>[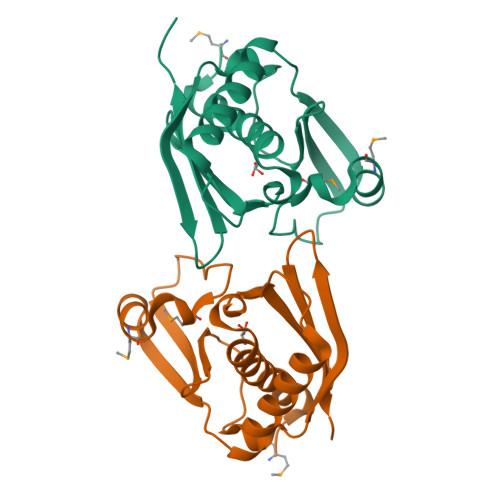2x]MYSIEVRTHSALHVVKGAVVKVLGSEAKWTYSTYVKGNKGVLIVKFDRKPSDEEIREIERLANEKVKENAPIKIYELPREEAEKMFGEDMYDLFPVPEDVRILKVVVIEDWNVNACNKEHTKTTGEIGPIKIRKVRFRKSKGLLEIHFELLELENPSLEHHHHHH>AQPTESEKEIYNQVNVVLKDAEGILEDLQSYRGAGHEIREAIQHPADEKLQEKAWGAVVPLVGKLKKFYEFSQRLEAALRGLLGALTSTPYSPTQHLEREQALAKQFAEILHFTLRFDELKMTNPAIQNDFSYYRRTLSRMRINNVPAEGENEVNNELANRMSLFYAEATPMLKTLSDATTKFVSENKNLPIENTTDCLSTMASVCRVMLETPEYRSRFTNEETVSFCLRVMVGVIILYDHVHPVGAFAKTSKIDMKGCIKVLKDQPPNSVEGLLNALRYTTKHLNDETTSKQIRSMLQ[2x]

Rac1 is a major regulator of actin dynamics, with GTP-bound Rac1 promoting actin assembly via the Scar/WAVE complex. CYRI competes with Scar/WAVE for interaction with Rac1 in a feedback loop regulating actin dynamics. Recently, a novel effector of Rac1, Fam49B also known as CYRI-B (CYFIP-related Rac interactor), has been reported to bind to active Rac1 and oppose the activation of the Scar/WAVE complex (Fort et al., 2018). CYRI-B, its isoform CYRI-A and the Scar/WAVE complex all possess an evolutionarily conserved Rac1 binding domain (RBD) termed the DUF1394 domain.

To obtain crystals capable of diffracting to high resolution, the N-terminal residues (1–25) involved in membrane binding were truncated, but the entire DUF1394 domain (residues 26–324) was retained. The structure of each CYRI-BΔN monomer consists of 12 alpha helices packed into two bundles running perpendicular to each other to produce an L-shape fold. Based on the structural alignment, we define CYRI-B DUF1394 domain as a module comprising two helical bundles in an L-shape fold. The asymmetric unit contains two molecules of CYRI-BΔN with each monomer “slotting” against the other to form a compact dimer. The dimer interface produces a large contact area of 1524Å2, yet there are relatively few bonding contacts between the CYRI monomers. Briefly, R161 form a hydrogen bond with A192, R165 and M166 binds to Q324, I168 with R320, N169 with S321 and Q324. Thus to test if the CYRI-B dimer observed in the asymmetric unit can occur in solution and if it can heterodimerize with CYRI-A, we used pulldown assays, which revealed a weak but reproducible interaction between MBP-CYRI-A or CYRI-B with HA-CYRI-B. Overlaying CYRI-BΔN:Rac1Q61L complex structure with that of the CYRI dimer, we can see that the two directly compete for the same binding interface. This raises the possibility that CYRI dimers autoinhibit Rac1 binding and regulate CYRI functionality. The crystal structure of CYRI-BΔN reveals the presence of an autoinhibited dimer present in solution and in cells as revealed through pulldowns and PLA.> GAGCAGACTAGACACCACTCA;> TGTCT;> TCTGAGTGG;>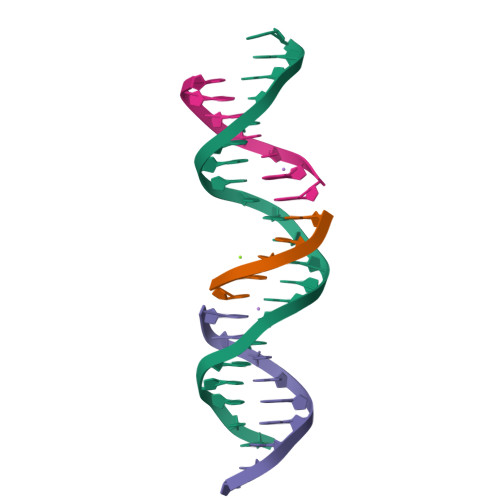 AGTCTGC>[4x]MRIVPFGAAREVTGSAHLLLAGGRRVLLDCGMFQGKEEARNHAPFGFDP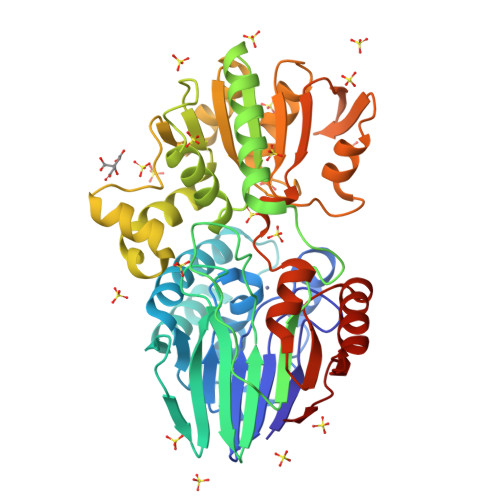KEVDAVLLTHAALDHVGRLPKLFREGYRGPVYATRATVLLMEIVLEDALKVMDEPFFGPEDVEEALGHLRPLEYGEWLRLGALSLAFGQAGHLPGSAFVVAQGEGRTLVYSGDLGNREKDVLPDPSLPPLADLVLAEGTYGDRPHRPYRETVREFLEILEKTLSQGGKVLIPTFAVERAQEILYVLYTHGHRLPRAPIYLDSPMAGRVLSLYPRLVRYFSEEVQAHFLQGKNPFRPAGLEVVEHTEASKALNRAPGPMVVLAGSGMLAGGRILHHLKHGLSDPRNALVFVGYQPQGGLGAEIIARPPAVRILGEEVPLRASVHTLGGFSGHAGQDELLDWLQGEPRVVLVHGEEEKLLALGKLLALRGQEVSLARFGEGVPV> ATFEIVNRCSYTVWAAASKGNAALDAGGRQLNSGESWTINVEPGTNGGK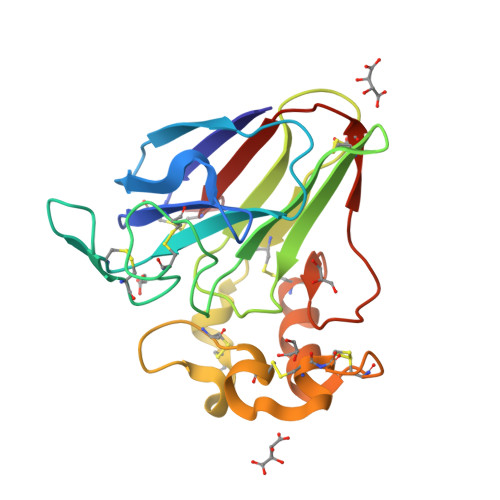IWARTDCYFDDSGSGICKTGDCGGLLRCKRFGRPPTTLAEFSLNQYGKDYIDISNIKGFNVPMDFSPTTRGCRGVRCAADIVGQCPAKLKAPGGGCNDACTVFQTSEYCCTTGKCGPTEYSRFFKRLCPDAFSYVLDKPTTVTCPGSSNYRVTFCPTA> SNAMNKQIDLPIADVQGSLDTRHIAIDRVGIKAIRHPVVV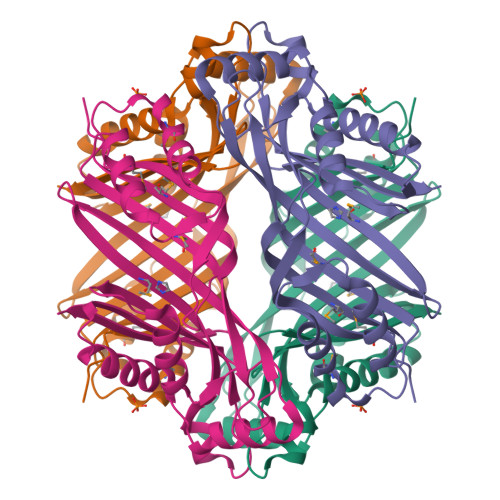ADKGGGSQHTVAQFNMYVNLPHNFKGTHMSRFVEILNSHEREISVESFEEILRSMVSRLESDSGHIEMAFPYFINKSAPVSGVKSLLDYEVTFIGEIKHGNQYSFTMKVIVPVTSLCPCSKKISDYGAHNQRSHVTISVRTNSFIWIEDIIRIAEEQASCELYGLLKRPDEKYVTERAYNNPKFVEDIVRDVAEVLNHDDRIDAYIVESENFESIHNHSAYALIERDKRIR> MSHHHHHHASERLPNRPACLLVASGAAEGVSAQSFLHCFTMASTAFNLQVATPGGKAMEFVDVTESNARWVQDFRLKAYASPAKLESIDGARYHALLIPSCPGALTDLASSGSLARILQHFHSESKPICAVGHGVAALCCATNEDRSWVFDSYSLTGPSVCELVRAPGFARLPLVVEDFVKDSGA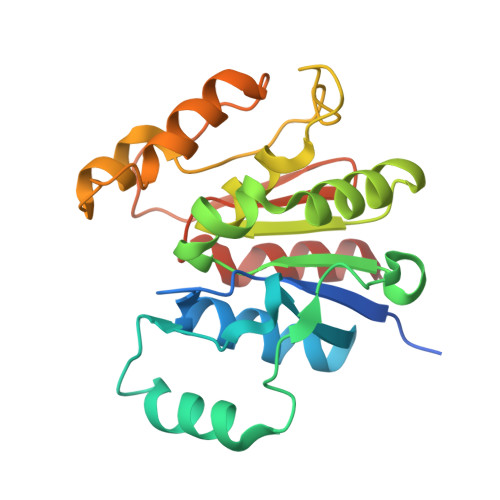CFSASEPDAVHVVLDRHLVTGQNASSTVPAVQNLLFLCGSRK> MGLLDRLSGLLGLKKKEVHVLCLGLDNSGKTTIINKLKPSNAQSQDIVPTIGFSIQKFKSSSLSFTVFDMSGQGRYRNLWEHYYKEGQAIIFVIDSSDKLRMVVAKEELRTLLNHPDIKHRRIPILFFANKMDLRDALTSVKVSQLLCLEDIKDKPWHICASDAIKGEGLQEGVDWLQDQIQSVKT;> MLQPVFTLKLRHKISPRMVAVGRYDGTHPCLAAATQAGKVFIHNPHSRSQHLGAPRVLQSPLESDVSLLNINQTVSCLTAGVLNPELGYDALLVGTQTNLLAYDVYNNSDLFYREVADGASAIVLGTLGDITSPLAIIGGNCALQGFNHEGNDLFWTVTGDNVHSLALCDFDGDGKKELLVGSEDFDIRVFKEDEIVAEMSETEIITSLCPMYGSRFGYALSNGTVGVYDKTARYWRIKSKNQAMSIHAFDLNSDGVCELITGWSNGKVDARSDRTGEVIFKDNFSSAIAGVVEGDYRMEGCQQLICCSVDGEIRGYLPGTAEMRGNLMDISVEQDLIRELSQKKQNLLLELRNYEENAKAELSSPLNEADGHRGVIPANTKHHTALSVSLGSEAQAAHAELCISTSNDTIIRAVLIFAEGVFAGESHVVHPSVHHLSSSVRIPITPPKDIPVDLHLKTFVGYRSSTQFHVFELTRQLPRFSMYALTSPDPASEPLSYVNFIIAERAQRVVMWLNQNFLLPEDTNIQNAPFQVCFTSLRNGGQLYIKIKLSGEITVNTDDIDLAGDIIQSMASFFAIEDLQVEADFPVYFEELRKVLVKVDEYHSVHQKLSADMADNSNLIRSLLVQAEDARLMRDMKTMKNRYKELYDLNKDLLNGYKIRCNNHTELLGSLKAVNQAIQRAGHLRVGKPKNQVITACRDAIRSNNINMLFRIMRVGTASS;> MDLNLNRADYLQVGVTSQKTMKLLPASKHRATQKVVVGDHDGIVMCFGMKKGEAVTVFKTLPGQKIARLELGGALNTPQEKIFIAAGSEIRGFTKRGKQFLSFETNLTESIKAMHISGSDLFLSASYIYNHYCDCKDQHYYLSGDKINDVICLPVERLLREVPVLACQDRVLRVLQGSDVTYEIEVPGPPTVLALHNGNGGDSGEDLLFGTSDGKLGLIQITTSKPIHKWEIRNEKKRGGILCVDSFDIVGDGVKDLLVGRDDGMVEVYGFDNANEPVLRFDHTLSESVTSIQGGCVGKDGYDEIVVSTYSGWITGLTTEPVHKESGPGEELKFNQEMQNKISSLRSELEQLQYKVLQEREKYQQSSQSSKAKSAVPSFSVNDKFTLNKDDASYSLILEVQTAIDNVLIQSDVPIDLLDVDKNSAVVSFSSCDSESNDNFLLATYRCQANTTRLELKIRSIEGQYGTLQAYVTPRIQPKTCQVRQYHIKPLSLHQRTHFIDHDRPMNTLTLTGQFSFSELHSWVVFCMPEVPEKPPAGECVTFYFQNTFLDTQLESTYRKGEGVFKSDNISTISILKDVLSKEATKRKINLNISYEINEVSVKHTLKLIHPKLEYQLLLAKKVQLIDALKELQVHEGNTNFLIPEYRCILEEADHLQEEYKKQPAHLERLYGMITDLFIDKFKFKGTNVKTKVPLLLEILDSYDQNALIAFFDAA;> MAATSSSDSDGGKGESEANSKWLDSLSDSMANIHTFSACLALADFHGDGEYKLAMGDLGPDGRQPRLKVLKGHTLVSQKPLPDLPAAAVTFLMASHEPRTPALAIASGPCVYVYKNLKPYFKFSLPSLPTNPLEQDLWNQAKEDQIDPLTLKEMLEGIREKAEVPLSVQSLRFLPLELSEMEAFVNQHKSKSIRRQTVITTMTTLKKNLADEDAVSCLVLGTENKELLVLDPEAFTILAKMSLPSVPAFLEASGQFDVEFRLAAACRNGSIYILRRDSKRPKYCIELGAQPVGLVGVHKVLVVGSNQDSLHGFTYKGKRLWTVQMPAAILAMNLLEQHSRGLQAVMAALANEEVRIYHDKVLLNVIRTPEAVTSLCFGRYGREDNTLIMTTLGGGLIIKILKRTAVFAEGGGEAGPPPSQAIKLNVPRKTRLYVDQTLREREAGTAMHRTFQADLYLLRLRAARAYVQALESSLSPVSLTAREPLKLHAVVQGLGPTFKLTLHLQNTSTARPILGLVVCFLYNEVLYALPRAFFKVPLLVPGLNYPLETFVKSLSDKGISDIIKVLVLREGQSTPLLSAHINMPMSEGLAAD;> MAEEKLSARTQLPVSAESQKPVLKKAPEFPILEKQNWLIHLYYIQKDYEACKAVIKEQLQETHGLCEYAIYVQALIFRLEGNIQESLRLFQMCAFLSPQCADNLKQVARSLFLLGKHKAAIEVYNEAAKLNQKDWEICHNLGVCYIYLKQFDKAQDQLHNALHLNRHDLTYIMLGKIFLLKGDLDKAIEIYKKAVEFSPENTELLTTLGLLYLQLGIYQKAFEHLGNTLTYDPTNYKAILAAGSMMQTHGDFDVALTKYKVVACAVIESPPLWNNIGMCFFGKKKYVAAISCLKRANYLAPLDWKILYNLGLVHLTMQQYASAFHFLSAAINFQPKMGELYMLLAVALTNLEDSENAKRAYEEAVRLDKCNPLVNLNYAVLLYNQGEKRDALAQYQEMEKKVNLLKYSSSLEFDPEMVEVAQKLGAALQVGEALVWTKPVKDPKSKHQTASTSKAAGFQQPLGSNQALGQAMSSAATCRKLSSGAGGTSQLTKPPSLPLEPEPTVEAQPTEASAQTREK;> MEPLLLAWSYFRRRRFQLCADLCTQMLEKSPCDQAAWILKARALTEMVYVDEIDVDEEGIAEMILDENAIAQVPRPGTSLKLPGTNQTGGPSPAVRPVTQAGRPITGFLRPSTQSGRPGTIEQAIKTPRTAYTARPIASSSGRFVRLGTASMLTSPDGPFINLSRLNLAKYAQKPKLAKALFEYIFHHENDVKTALDLAALSTEHSQYKDWWWKVQIGKCYYRLGLYREAEKQFKSALKQQEMVDTFLYLAKVYISLDQPLTALNLFKQGLDKFPGEVTLLCGIARIYEEMNNISSATEYYKEVLKQDNTHVEAIACIGSNHFYTDQPEVALRFYRRLLQMGVYNCQLFNNLGLCCFYAQQYDMTLTSFERALSLAENEEEVADVWYNLGHVAVGTGDTNLAHQCFRLALVSNNQHAEAYNNLAVLEMRRGHVEQAKALLQTASSLAPHMYEPHFNFATISDKIGDLQRSYAAAKKSEAAFPDHVDTQHLIKQLEQHFAML;> MSVLDALWEDRDVRFDVSSQQMKTRPGEVLIDCLDSVEDTKGNNGDRGRLLVTNLRIVWHSLALPRVNLSIGYNCILNITTRTANSKLRGQTEALYVLTKCNSTRFEFIFTNLVPGSPRLYTSLIAVHRAYETSKMYRDFKLRSALIQNKQLRLLPQENVYNKINGVWNLSSDQGNLGTFFITNVRIVWHANMNDSFNVSIPYLQIRSVKIRDSKFGLALVIESSQQSGGYVLGFKIDPVEKLQESVKEINSLHKVYSANPIFGVDYEMEEKPQPLEALTVKQIQDDVEIDSDDHTDAFVAYFADGNKQQDREPVFSEELGLAIEKLKDGFTLQGLWEVMN;> MAETKSMFREVLPKQGQLYVEDITTMVLCKPKL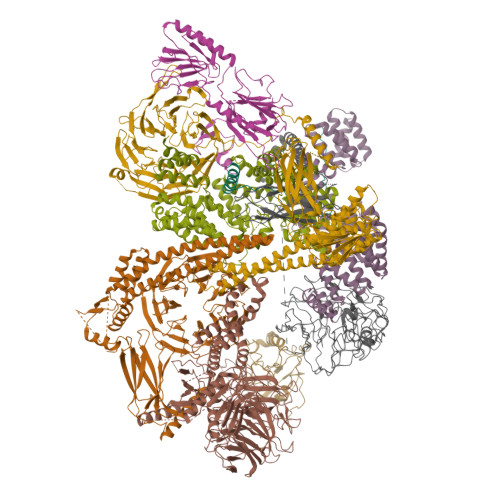LPLKSLTLEKLEKMQQAAQDTIHQQEMTEKEQKITH;> MSLFKARDWWSTVLGDKEEFDQGCLCLADVDNTGNGQDKIIVGSFMGYLRIFNPHPVKTGDGAQAEDLLLEVHLRDPILQVEVGKFVSGTEMLHLAVLHSRKLCVYSVSGTLGNVEHGNQYQIKLMYEHNLQRTACNMTYGSFGGVKGRDLICIQSVDGMLMVFEQESYAFGRFLPGSLLPGPLAYSSRTDSFITVSSCHQVESYKYQVLAFATDADKRQETEQQKHGSGKRLVVDWTLNIGEQAIDICIVSFIQSASSVFVLGERNFFCLKDNGQIQFMKKLDYSPSCFLPYCSVSEGTINTLIGNHNNMLHIYQDVTLKWATQLPHVPVAVRVGCLHDLKGVIVTLSDDGHLQCSYLGTDPSLFQAPKVESRELNYDELDMELKELQKVIKNVNKSQDVWPLTEREDDLKVSAMVSPNFDSVSQATDVEVGADLVPSVTVKVTLKNRVALQKIKLSIYVQPPLVLTGDQFTFEFMAPEMTRTVGFSVYLKGSYSPPELEGNAVVSYSRPTERNPDGIPRVSQCKFRLPLKLVCLPGQPSKTASHKLTIDTNKSPVSLLSLFPGFAKQSEDDQVNVMGFRFLGGSQVTLLASKTSQRYRIQSEQFEDLWLITNELIIRLQEYFEKQGIKDFTCSFSGSVPLEEYFELIDHHFELRINGEKLEELLSERAVQFRAIQRRLLTRFKDKTPAPLQHLDTLLDGTYKQVIALADAVEENQDNLFQSFTRLKSATHLVILLIGLWQKLSADQIAILEAAFLPLQQDTQELGWEETVDAALSHLLKTCLSKSSKEQALNLNSQLGIPKDTSQLKKHITLFCDRLAKGGRLCLSTDAAAPQTMVMPGGCATIPESDLEGRSIDQDSSELFTNHKHLMVETPVPEVSPLQGVTE> HHHHHHFNLPPGNYKKPVLLKSTETGQYLRINPDGTVDGTRDRSDVHIQFQISPEGNGEVLLKSTETGQYLRINPDGTVDGTRDRSDVHIQFQI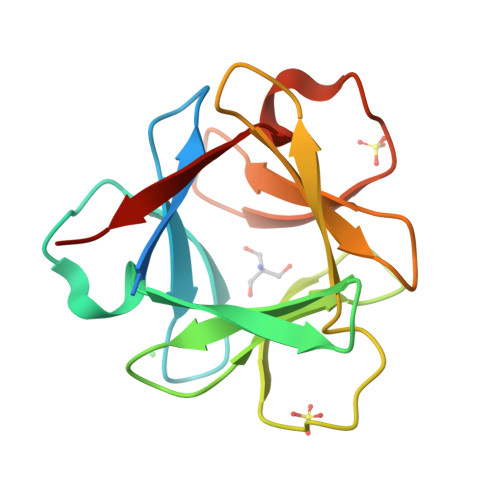SPEGNGEVLLKSTETGQYLRINPDGTVDGTRDRSDVHIQFQISPEGNG> APRFGGVMRPN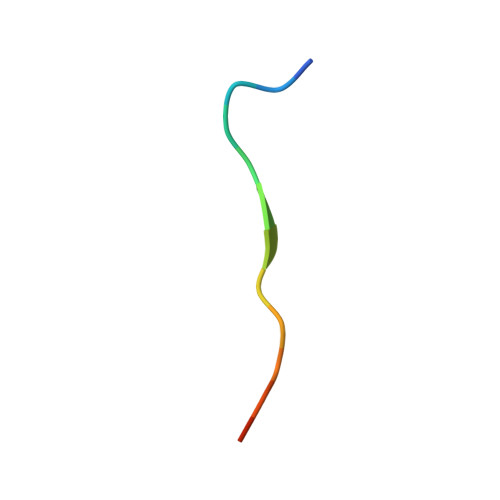RYR> MASGSVLTAIDNDKVAVGDKVTLTINVDKITNFSGYQFNIKYNTTYLQPWDTIADEAYTDSTMPDYGTLLQG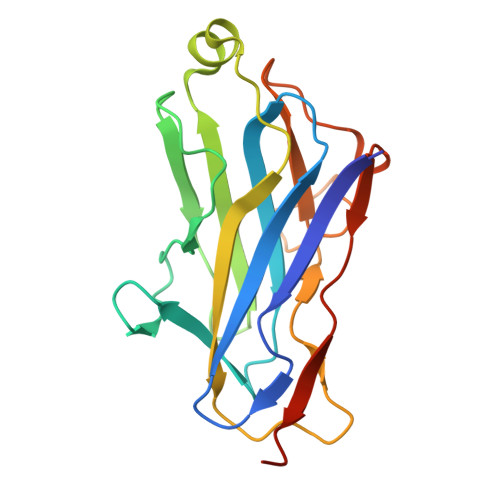RFNATDMSKHNLSQGVLNFGRLYMNLSAYRASGKPESTGAVAKVTFKVIKEIPAEGIKLATFENGSSMNNAVDGTMLFDWDGNMYSSSAYKVVQPGLIYPKLEHHHHHH6-{[(3R,4R)-4-(2-{[(2R)-1-(3-fluorophenyl)propan-2-yl]amino}ethoxy)pyrrolidin-3-yl]methyl}-4-methylpyridin-2-amine 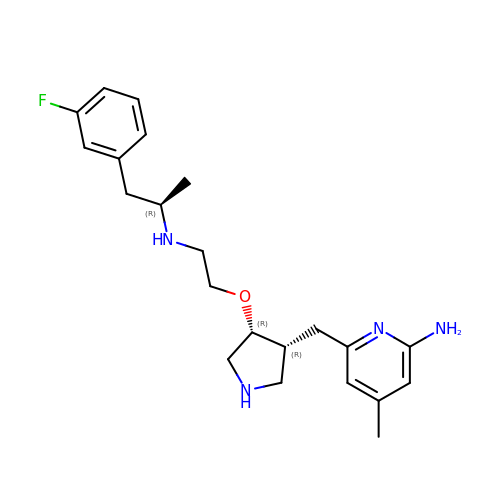| C22 H31 F N4 O | AUSIEXNWJKDTQY-BLIXFSHQSA-N> GAMDPEFTLSSEKKAKKVRFYRNGDRYFKGIVYAISPDRFRSFEALLADLTRTLSDNVNLPQGVRTIYTIDGLKKISS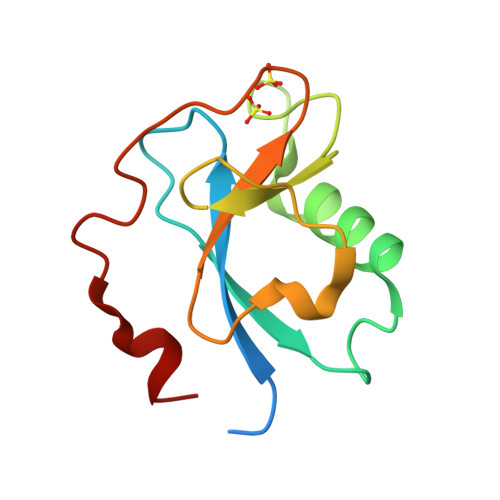LDQLVEGESYVCGSIEPFKKLEYTKNVNPNWSVNV> MAKVRIYQLAKELGMETQELLELLDQMGVAYKSHASTLEEKDAEAVRELVKEQRGLQEKLAEEERRKSLPRRPPVVVIMGHVDHGKTTLLDYLRKSRIAEKEAGGITQHVGAFEVKTPQGTVVFIDTPGHEAFTTIRQRGAKVADIAVIVIAADDGIMPQTEEAIAHAKAAGAKLIFAINKIDLPQADPEKVKRQLMERGFVPEEYGGDAIVIPISAKTGQGVQDLLEMILLLAELEDYRADPNAEPRGVILESKLDKQAGIIANMLVQEGTFRVGDYVVAGEAYGRIRAMMDADGNQRKEAGPGSAVQVLGFQELPHAGDVVEWVPDLEAAKEIAEERKEERKAREEEEKARRPRTMAELLR

Translation initiation factor 2 (IF2) is involved in the early steps of bacterial protein synthesis. It promotes the stabilization of the initiator tRNA on the 30S initiation complex (IC) and triggers GTP hydrolysis upon ribosomal subunit joining. IF2 is also responsible for the fast subunit association and 70S IC formation, an event that is directly coupled to the activation of the IF2 GTPase. Here, we present the crystal structure of the eubacterial IF2 core as the individual apoprotein and in GTP-bound and GDP-bound forms.

Comparison of the GTP and GDP complexes of IF2 reveals several significant differences within the nucleotide-binding site. The largest conformational changes are observed for residues located around the γ-phosphate group. The Val82 side chain, which moves strongly upon nucleotide binding in order to comply with reasonable van der Waals distances to the γ-phosphate, rotates slightly between the GTP-bound and GDP-bound states. Upon GTP hydrolysis and phosphate release Lys86 releases its hydrogen bond to the GTP γ-phosphate and becomes available for interaction with His130. However, it is striking that the histidine adopts two nucleotide-dependent conformations. In the presence of GTP His130 is rotated away from the nucleotide, clearly in order to avoid uncontrolled GTP hydrolysis occurring; in the GDP-bound state Lys86 occupies the place of the GTP γ-phosphate and forms a hydrogen bond to His130. It is therefore likely that when activated by the 50S ribosomal subunit in the full ribosome context His130 adopts a conformation similar to that observed in the GDP complex, in which it is perfectly positioned to activate the water molecule located next to the γ-­phosphate.Acetyl-CoA synthetase (Acs) generates acetyl-coenzyme A (Ac-CoA) but its excessive activity can deplete ATP and lead to a growth arrest. To prevent this, Acs is regulated through Ac-CoA-dependent feedback inhibition executed by Ac-CoA-dependent acetyltransferases such as AcuA in Bacillus subtilis. AcuA acetylates the catalytic lysine of AcsA turning the synthetase inactive. Acs enzymes consists of two consecutively operating modules, a C-terminal domain (CTD) catalyzing the first and a N-terminal domain (NTD) for the second reaction step.

A second major class of particles showed the AcsA homodimer bound to AcuA. In these particles, the CTD of the AcsA subunit of the homodimer bound to AcuA was resolved, while the CTD of the non-AcuA-bound AcsA subunit in the homodimer remained unresolved. Our structure clearly demonstrates that AcuA restricts the conformational flexibility of the CTD, thereby enforcing a so far unreported conformation of the NTD and CTD of AcsA. AcsA and AcuA contribute 1,859.8 Å2 and 1,861.9 Å2 of solvent accessible area, respectively, to the interface of the complex. First, the very C-terminus of AcuA (amino acids 203 – 210) reaches out into the active site of the AcsA NTD. A detailed analysis revealed that the main chains of AcuA_M209 and Y208 form hydrogen bonds with AcsA_D255, while the main chain of AcuA_Y210 forms a hydrogen bond with AcsA_R108. Additionally, a loop containing the catalytic residue K549 within the CTD of AcsA aligns with the active site of AcuA. The cryo-EM structure of the complex shows that the very C-terminus of AcuA inserts into the CoA-binding site of the NTD of AcsA. The AcsA domain arrangement enforced by the binding of AcuA appears unsuitable for a productive synthesis of Ac-CoA catalyzed by AcsA and may thus be considered as the “locked” state.

>[2x]MNLKALPAIEGDHNLKNYEETYRHFDWAEAEKHFSWHETGKLNAAYEAIDRHAESFRKNKVALYYKDAKRDEKYTFKEMKEESNRAGNVLRRYGNVEKGDRVFIFMPRSPELYFIMLGAIKIGAIAGPLFEAFMEGAVKDRLENSEAKVVVTTPELLERIPVDKLPHLQHVFVVGGEAESGTNIINYDEAAKQESTRLDIEWMDKKDGFLLHYTSGSTGTPKGVLHVHEAMIQQYQTGKWVLDLKEEDIYWCTADPGWVTGTVYGIFAPWLNGATNVIVGGRFSPESWYGTIEQLGVNVWYSAPTAFRMLMGAGDEMAAKYDLTSLRHVLSVGEPLNPEVIRWGHKVFNKRIHDTWWMTETGSQLICNYPCMDIKPGSMGKPIPGVEAAIVDNQGNELPPYRMGNLAIKKGWPSMMHTIWNNPEKYESYFMPGGWYVSGDSAYMDEEGYFWFQGRVDDVIMTSGERVGPFEVESKLVEHPAIAEAGVIGKPDPVRGEIIKAFIALREGFEPSDKLKEEIRLFVKQGLAAHAAPREIEFKDKLPKTRSGKIMRRVLKAWELNLPAGDLSTMED;> MEHHKTYHSANIKTATGSLLIEGPVSPEDLAGYEFHKDLTAFRPPREQHEALVDIAGLPEGRIIIARDGRTIVGYVTYLYPDPLERWSEGNMEDLIELGAIEVAPDYRGCAVGKTLLTVSMMDEQMENYIVMTTEYYWHWDLKGMKKDVWEYRKIMEKMMNAGGLVWFATDEPEISSHPANCLMARIGKNVSQESIEQFDRLRFYHRYMY>[2x]MILVFLGPPGAGKGTQAKRLAKEKGFVHISTGDILREAVQKGTPLGKKAKEYMERGELV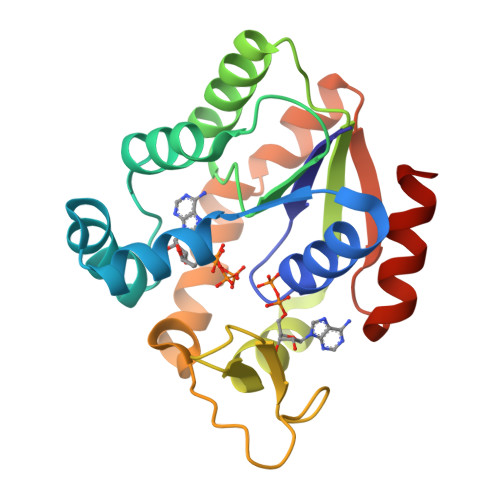PDDLIIALIEEVFPKHGNVIFDGFPRTVKQAEALDEMLEKKGLKVDHVLLFEVPDEVVIERLSGRRINPETGEVYHVKYNPPPPGVKVIQREDDKPEVIKKRLEVYREQTAPLIEYYKKKGILRIIDASKPVEEVYRQVLEVIGDGN>[3x]GSHMVHHPPSYVAHLASDFGVRVFQQVAQASKDRNVVFSPYGVASVLAMLQLTTGGETQQQIQAAMGFKIDDKGMAPALRHLYKELMGPWNKDEISTTDAIFVQRDLKLVQGFMPHFFRLFRSTVKQVDFSEVERARFIINDWVKTHTKGMISNLLGKGAVDQLTRLVLVNALYFNGQWKTPFPD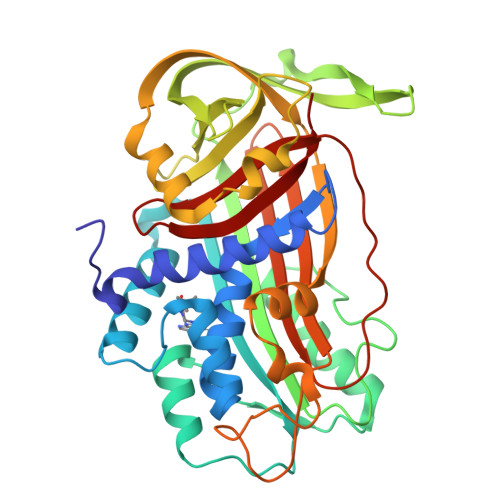SSTHRRLFHKSDGSTVSVPMMAQTNKFNYTEFTTPDGHYYDILELPYHGDTLSMFIAAPYEKEVPLSALTNILSAQLISHWKGNMTRLPRLLVLPKFSLETEVDLRKPLENLGMTDMFRQFQADFTSLSDQEPLHVAQALQKVKIEVNESGTVASSSTAVIVSARMAPEEIIMDRPFLFVVRHNPTGTVLFMGQVMEP>[2x]MFNRTTQLKSKHPCSVCTRRKVKCDRMIPCGNCRKRGQDSECMKSTKLITASSSKEYLPDLLLFWQNYEYWITNIGLYKTKQRDLTRTPANLDTDTEECMFWMNYLQKDQSFQLMNFAMENLGALYFGSIGDISELYLRVEQYWDRRADKNHSVDGKYWDALIWSVFTMCIYYMPVEKLAEIFSVYPLHEYLGSNKRLNWEDGMQLVMCQNFARCSLFQLKQCDFMAHPDIRLVQAYLILATTTFPYDEPLLANSLLTQCIHTFKNFHVDDFRPLLNDDPVESIAKVTLGRIFYRLCGCDYLQSGPRKPIALHTEVSSLLQHAAYLQDLPNVDVYREENSTEVLYWK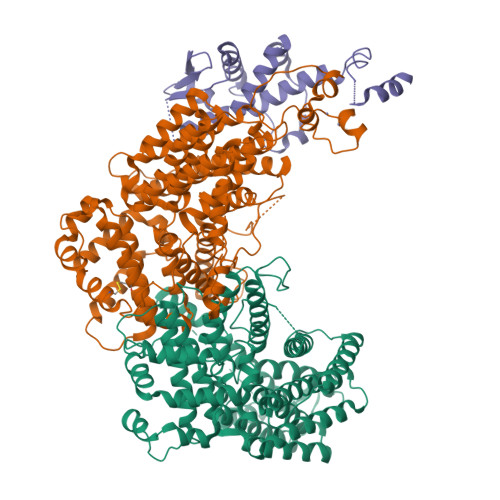IISLDRDLDQYLNKSSKPPLKTLDAIRRELDIFQYKVDSLEEDFRSNNSRFQKFIALFQISTVSWKLFKMYLIYYDTADSLLKVIHYSKVIISLIVNNFHAKSEFFNRHPMVMQTITRVVSFISFYQIFVESAAVKQLLVDLTELTANLPTIFGSKLDKLVYLTERLSKLKLLWDKVQLLDSGDSFYHPVFKILQNDIKIIELKNDEMFSLIKGLGSLVPLNKLRQESLLEEEDENNTEPSDFRTIVEEFQSEYNISDILSGSGGSGENLYFQ;> MVTSNVVLVSGEGERFTVDKKIAERSLLLKNYLNDMHDSNLQNNSDSESDSDSETNHKSKDNNNGDDDDEDDDEIVMPVPNVRSSVLQKVIEWAEHHRDSNFPDEDDDDSRKSAPVDSWDREFLKVDQEMLYEIILAANYLNIKPLLDAGCKVVAEMIRGRSPEEIRRTFNIVNDFTPEEEAAIRRENEWAEDR GapR (growth-associated A/T-binding protein involved in regulation) is a chromosome structure protein conserved in α-proteobacteria, and it is discovered initially as an essential nucleoid-associated protein for normal growth and cell division in Caulobacter crescentus (1–3). Depletion of GapR gene in Caulobacter cells results in severe defects in cell growth, cell division, cell size, DNA replication, chromosome segregation/condensation and gene expression. Our current studies clearly demonstrate that free GapR is a tetramer, but not a dimer. Taken all together, there exist both major conformation and minor conformation for free GapR in solution, which are in dynamic exchange equilibrium with each other.

We report the crystal structure of a 10-bp A-tract DNA bound by GapR in an open tetrameric conformation, which is representative of the minor conformers of free GapR. In this crystal structure, each protomer of GapR is consisted of two α-helices (α1: residues 13–51; α2: residues 55–89) that adopt a V-shape conformation. The open tetramer of GapR can be considered as a dimer of two antiparallel coiled-coil dimer-units formed mainly through α1 helices. The two dimer-units form a tetramer through further dimerization with one α2 helix from each dimer-unit in an antiparallel coiled-coil conformation, while the other two α2 helices are free of contact. The tetrameric interface is formed by hydrophobic residues V57, V61, I64, I78, L81 and Y82, with 6 intermolecular salt bridges between residues K60 and E74, R63 and E74, D68 and K71. The 10A DNA is partially wrapped inside the open tetramer of GapR, which adopts a C-clamp like shape. The binding of 10A DNA is mainly through electrostatic interactions between the phosphate groups of a 15-bp DNA portion and side-chains of positively charged residues of GapR, consisting of K34, K49, K59 and R63 of all four protomers, K42 and K60 from three of the protomers, and K56 and K66 from two of the protomers, according to interface analysis using PISA. There are no base-specific contacts between GapR and 10A DNA. Therefore, the major difference between the two tetramer structures lies that one tetrameric interface of the closed conformation is fully dissociated in the open tetrameric conformation, while the other one is rearranged to form a new antiparallel coiled-coil interface. Therefore, the crystal structure of the open tetrameric GapR should be considered as representative of an ensemble of dynamic minor conformations, which should be in fast exchange on the NMR time scale.

>MADDAIPHTDVLNSTAQGQLKSIIERVERLEVEKAEIMEQIKEVYAEAKGNGFDVKVLKKVVRIRKQDRAKRQEEDAILDLYLSAIGEILEHHHHHH[4x]> SFDFKDTDMKRLDMEIEKEKVEYMEKSKHLQEQLNELKTEIEALKLKERETALDILHNENSD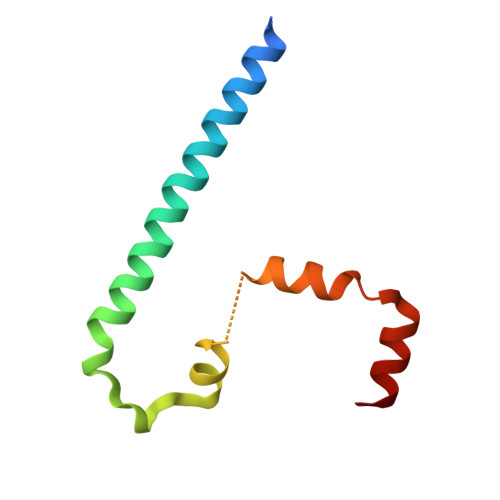RGGSSKHNTIKKLTLQSWKSRVAFFEEL>GPGSEVLDKDAVKKMFAVGTASLGHVPVLDVGRFSSEIAEARLALFQKQVEITKKHRGDANVRYAWLPAKREVLSAVMMQGLGVGGAFIR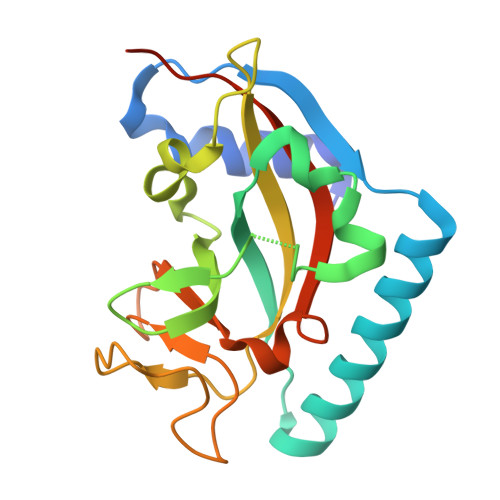KSIYGVGIHLTAADCPYFSARYCDVDENGVRYMVLCRVIMGNMELLRGDKAQFFSGGEEYDNGVDDIESPKNYIVWNINMNTHIFPEFVVRFKLSNLPNAEGNL[8x]> N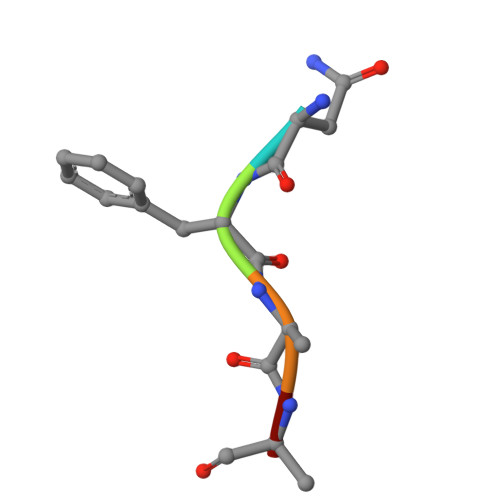FAAR>MVHYYRLSLKSRQKAPKIVNSKYNSILNIALKNFRLCKKHKTKKPVQILALLQEIIPKSYFGTTTNLKRFYKVVEKILTQSSFECIHLSVLHKCYDYDAIPWLQNVEPNLRPKLLLKHNLFLLDNIVKPIIAFYYKPIKTLNGHEIKFIRKEEYISFESKVFHKLKKMKYLVEVQDEVKPRGVLNIIPKQDNFRAIVSIFPDSARKPFFKLLTSKIYKVLEEKYKTSGSLYTCWSEFTQKTQGQIYGIKVDIRDAYGNVKIPVLCKLIQSIPTHLLDSEKKNFIVDHISNQFVAFRRKIYKWNHGLLQGDPLSGCLCELYMAFMDRLYFSNLDKDAFIHRTVDDYFFCSP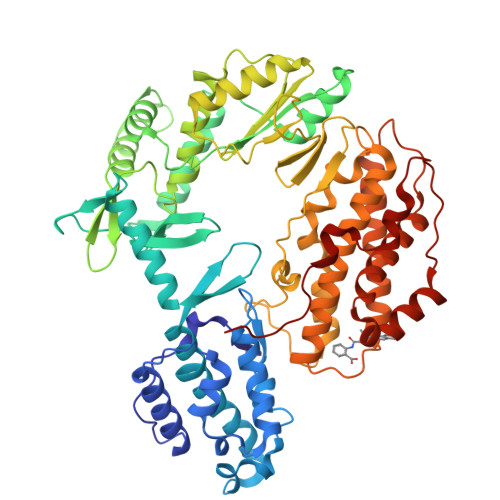HPHKVYDFELLIKGVYQVNPTKTRTNLPTHRHPQDEIPYCGKIFNLTTRQVRTLYKLPPNYEIRHKFKLWNFNNQISDDNPARFLQKAMDFPFICNSFTKFEFNTVFNDQRTVFANFYDAMICVAYKFDAAMMALRTSFLVNDFGFIWLVLSSTVRAYASRAFKKIVTYKGGKYRKVTFQCLKSIAWRAFLAVLKRRTEIYKGLIDRIKSREKLTMKFHDGEVDASYFCKLPEKFRFVKINRKASI[2x]>[6x]GSHMDQDSLSSSLKTCYKYLNQTSRSFAAVIQALDGEMRNAVCIFYLVLRALDTLEDDMTISVEKKVPLLHNFHSFLYQPDWRFMESKEKDRQVLEDFPTISLEFRNLAE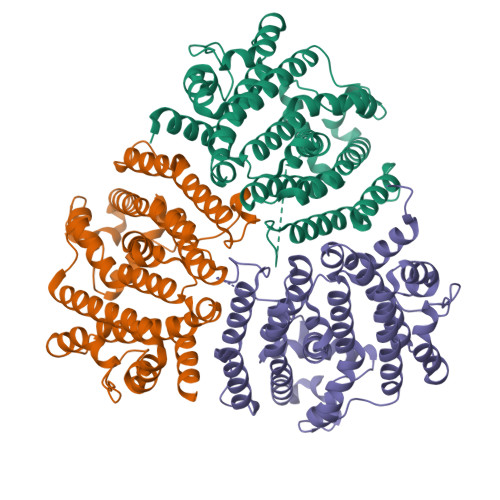KYQTVIADICRRMGIGMAEFLDKHVTSEQEWDKYCHYVAGLVGIGLSRLFSASEFEDPLVGEDTERANSMGLFLQKTNIIRDYLEDQQGGREFWPQEVWSRYVKKLGDFAKPENIDLAVQCLNELITNALHHIPDVITYLSRLRNQSVFNFCAIPQVMAIATLAACYNNQQVFKGAVKIRKGQAVTLMMDATNMPAVKAIIYQYMEEIYHRIPDSDPSSSKTRQIISTIRTQN>[2x]HMASKNVPSRAVKRVTAITKVEREAVLVCELPSFDVTDVEFDLFRARESTDKPLDVAAAIAYRLLLGSGLPQKFGCSDEVLLNFILQCRKKYRNVPYHNFYHVVDVCQTIHTFLYRGNVYEKLTELECFVLLITALVHDLDHMGLNNSFYLKTESPLGILSSASGNTSVLEVHHCNLAVEILSDPESDVFG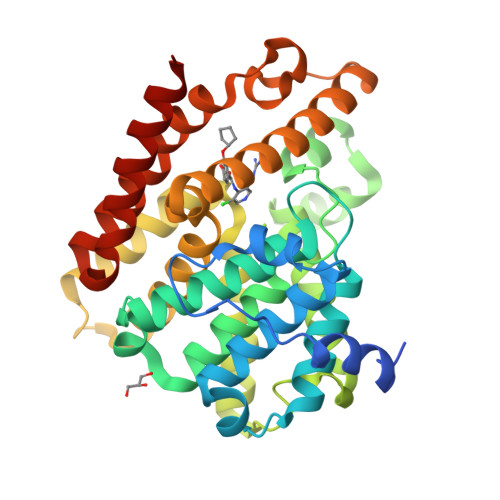GLEGAERTLAFRSMIDCVLATDMAKHGSALEAFLASAADQSSDEAAFHRMTMEIILKAGDISNVTKPFDISRQWAMAVTEEFYRQGDMEKERGVEVLPMFDRSKNMELAKGQIGFIDFVAAPFFQKIVDACLQGMQWTVDRIKSNRAQWERVLETR> MMRARRVVVALSPLAQLCVHVQWRLYTPIWQPDPAVDHVAPLRESDENRTLWASSAPIANVSDAIAAWIRFGNDPVLHTALPVIHAGQNERTRTDGSSASLSLSSLPSPSSTSPFATVEDYMGTNMVFGSPEHVKDSAAVWASYFERRYLSQLRHSRRTAANHVGLVNAPDVFTDEADRPETKWSQDTRFRERAYMAEKFLKEKVANLQQLEQALKQAKPAEYIAFHDALQQQTLTLIPLPSPSVWHYGGARRTQWAERFLPLSHEAQQFFTTVLAEDLKRAGDAPEKVLQKVAAVFAEVGKILLQRHRRCLGGREWSALAPHEKDEFCMKEVERWKQQVEVGEFDPPLDGDDDPTSTEWQSEHDAIMQLMTATIDGLSFSALEFWTHTIRCEEMETEHIHTEKRVRAISAAARRAMYDTTSYEAVLQGIVDAVAKGQLDMKAAGFKPHMNDIWCQLNYAKFGASTVTQHTTTARRQLNYFHAGLLKEVAATAALYYATKPLSSSLDYASPYKFRRSLVGLFSTYGVEMVYAVQRPLLFSAANLAKAEDLIRGVVKNVARPFGERRRAKLKQLRANHRRLATPVQGVVVSAVVSDLLESGADVSEAKKAEKMQESVTFWPLGARRVVSYDWPTPHFDALKRRVAAAGSAVTAQSTKEIQEIKRNAFVEVSLWRRVTAEETKQRRDAVEEETRRVADVVRTIPPLAQVQQYATSLYQRIEDAAPFPAATDNNAKSEQEDDESSWEFVVMLDDRVVLNANQAAELYLPYTDASGVPIPQGECRVRVRGFDVDVNPTLNPAFCSEAFSTPFQVFDAIPQLVQQFFGTAKPSVAEVSDIPSSKFIQFCAFLREAGLDVPVQCEFEAGQVLNAEGDVFMEYFLNLLRSDRFHRSCAQAGLTEMQRVIESSCRAHWEVHHPGANEAEWAEARRRVLDRAMEKEREWWFPNEMLDVTNMSPGSNHGLRLPMYPATVRYGRELCTLLAAEGQFDNNSGLSATCAVNGTGAAESITFSTGDHISSTFSMEEALAVAKGALRN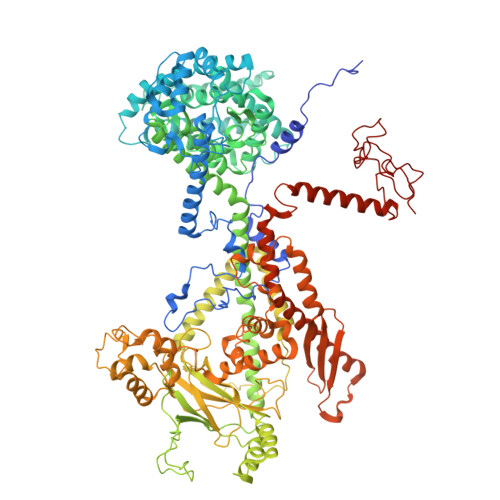AHDRQNTLAAFRLGPLSKHSQVLLFCGINATEFGGKYARTYTYAFEKAKKELAETFVSGRVVPGVDEDELLRVSDKEGVDRFASSTHPEQRKTQFVPRVGPGGAPIEDPTADQKTQWGR1-[(oxan-4-yl)methyl]piperazine 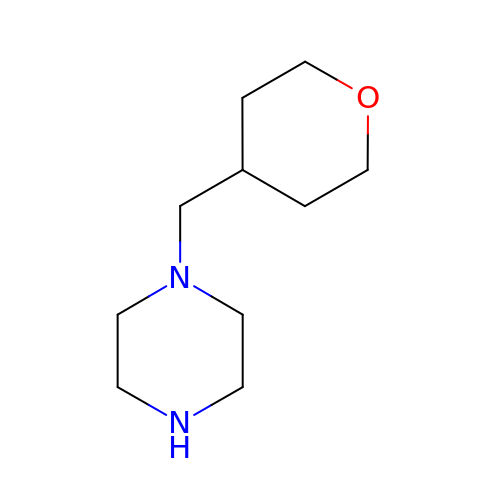| C10 H20 N2 O | XVQLGUIPBIHANF-UHFFFAOYSA-N>[2x]MTTGLSTAGAQDIGRSSVRPYLEECTRRFQEMFDRHVVTRPTKVELTDAELREVIDDCNAAVAPLGKTVSDERWISYVGVVLWSQSPRHIKDMEAFKAVCVLNCVTFVWDDMDPALHDFGLFLPQLRKICEKYYGPEDAEVAYEAARAFVTSDHMFRDSPIKAALCTTSPEQ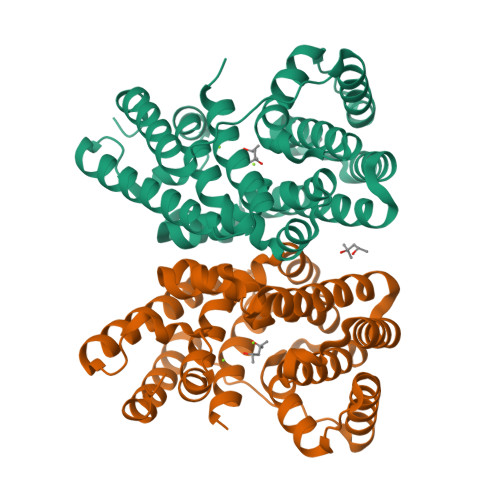YFRFRVTDIGVDFWMKMSYPIYRHPEFTEHAKTSLAARMTTRGLTIVNDFYSYDREVSLGQITNCFRLCDVSDETAFKEFFQARLDDMIEDIECIKAFDQLTQDVFLDLIYGNFVFTTSNKRYKTAVNDVNSRIQAAALEHHHHHH> GPTAAALERLTTEEVQGLSDVKTLVNQLYEALNVREHQLQKEVELTTQLETLQQELLPLEEKKLELEQVANRRSNWMAWAGLGLMSVQFGILARLTWWEYSWDIMEPVTY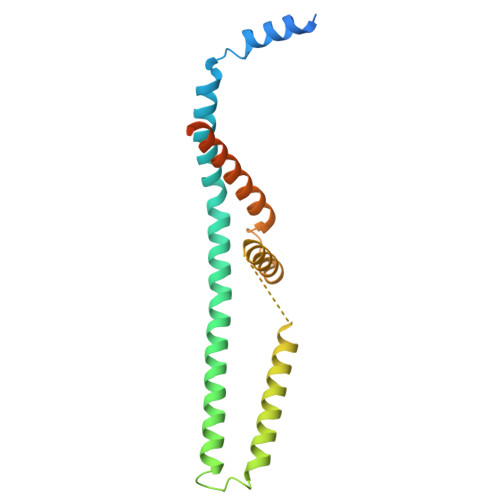FVTYGTAMAAYAYFVLTREEYILNDVRDRQQLLLLHKKAKKTGFDVNQYNVLKDQIAKLELDLKRLRDPLKLRLPPKAAAKEEGGWSHPQFEK> MGCFFSKRRKADKESRPENEEERPKQYSWDQREKVDPKDYMFSGLKDETVGRLPGTVAGQQFLIQDCENCNIYIFDHSATVTIDDCTNCIIFLGPVKGSVFFRNCRDCKCTLACQQFRVRDCRKLEVFLCCATQPIIESSSNIKFGCFQWYYPELAFQFKDAGLSIFNNTWSNIHDFTPVSGELNWSLLPEDAVVQDYVPIPTTEELKAVRVSTEANRSIVPISRGQRQKSSDESCLVVLFAGDYTIANARKLIDEMVGKGFFLVQTKEVSMK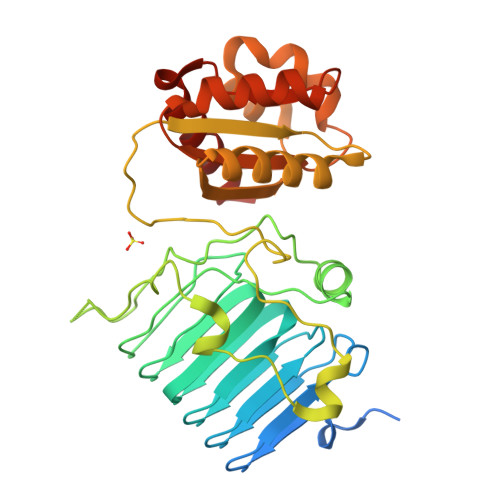AEDAQRVFREKAPDFLPLLNKGPVIALEFNGDGAVEVCQLIVNEIFNGTKMFVSESKETASGDVDSFYNFADIQMGI>GPLGSPEFREPLIATAVKFLQNSRVRQSPLATRRA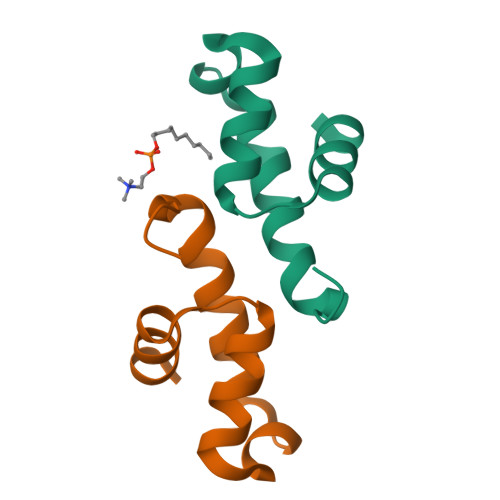FLKKKGLTDEEIDLAFQQS[2x]A recently found family of pore-forming toxins, called CDC-like proteins (CDCLs), are wide-spread in gut microbes and are a prevalent means of antibacterial antagonism. Analysis of the CDCLs belonging to the phylum Bacteroidota revealed the presence of sets of two-component CDCLs, one long CDCL (CDCLL) with four domains and one short CDCL (CDCLS) lacking the fourth C-terminal domain, that act as a bicomponent complex via a mechanism only previously observed in the mammalian complement MAC. Unlike CDCs, the CDCLs require proteolytic activation with both components containing a proteolytically cleavable activation loop critical to the regulation of pore formation. Here, we present the crystal structure of a proteolytically activated CDCLL and cryo–electron microscopy (cryo-EM) structures of a prepore-like intermediate and the transmembrane pore.

(A) The cryo-EM map at 2.87-Å resolution of the membrane-inserted pore complex, from focused refinement with C30 symmetry, reveals a β barrel pore with an outer diameter of 260 Å, an inner diameter of 167 Å, and a height of 105 Å. We modeled 30 subunits of EaCDCLS into the map, allowing a complete visualization of the membrane pore complex. This revealed the complete unfurling of the α-HBs to form the membrane-inserted TMHs that make up the β barrel pore, which is primarily hydrophilic and neither strongly positively nor negatively charged in the interior. Each EaCDCLS contributes four β strands, at a tilt of ~20 Å to the membrane normal, to yield a β barrel pore composed of 120 β strands stabilized by an extensive network of hydrogen bonds. As in the prepore-like oligomer, the HTH forms an interior α barrel, creating the narrowest portion of the pore. Comparison of the EaCDCLS protomer from the pore with the structure from the prepore state reveals no substantial changes beyond the TMH unfurling and further straightening of the core D3 β sheet. In contrast, the EaCDCL pore contains only 30 subunits with a substantially smaller pore inner diameter of ~167 Å. A major difference between our pore structure and the PLY pore structure is the smooth exterior of the EaCDCL pore, revealing full visualization of the β strands in the β barrel pore. Comparison of the various structures of EaCDCLS presented here reveals that the only change in height is due to unfurling of the α-HBs into the TMHs, while the D1 remains in the same position. However, we were unable to unambiguously visualize the EaCDCLL molecule, even after trialing various workflows incorporating symmetry expansion of particles, signal subtraction, focused refinement, 2D/3D classification, and 3D variability analysis of smaller wedges of the complex to extract the asymmetrical features provided by EaCDCLL.

>[30x]GSHMRQDSEVNPLQVQNSSKVLNPNVTLPANNLLYDEFFVSKESKLIEDSRNNKRKTSKIASLNPYASTKAVLTTTSSTLTSDQIVVTVPQKTFIGGVYNSTTLDNLDYTPISYPLDPITVSYSFPSDFIVDTIERPSLSSMRASVFKAMRAANFSGEQSLAFDYNIKQFSYYSELKIAFGSNVNIGKIFSIDISGSNNKIKRTTGVFAKFTQKNFTIDMDLPADGNIFKNNSDLALTNGKNPVYISSVTYGRLGIISIESNASYNEVNFALKAALTAGIVNGSLNIDSNSKKILEESDLSVYLVGGRGTDAVQVIKGFAGFSNFIVNGGQFTPEAPGVPIYFSASHASDNSVYYTTFTIDK>[2x]QGMQTLSSILRTIAPLDSKAMARATTRLDGLLKPQGSLGRLEQLAIQLAGMRGLYGHQVDRKQIIVMAADHGVYDEGVAISPRVVTMVQALNMVRGVTGVCVLAANAGAEVKIVDVGIDSDTLPGVIDMKVARGSGNIARGAAMTRQQAEDLLIASATLTLQQAAGGVKVFGVGELGMANTTPAAAMVSVFTDSDPELAVGIGANFP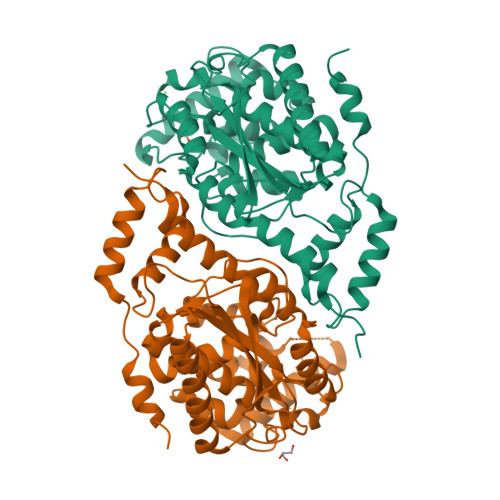SEQLHHKVAVVRRAIETNQPDASDGIDVLAKVGGFDLVGMTGVMLGAAAAGLPVVLDGFLSYASALAACRIEAKVRDYLIPSHLSAEKGAVIALNHLQLEPYLQMGMRLGEGSGAALAMHLVDAACAMYNNMGSLAESNIELPGCVN> PILEKAP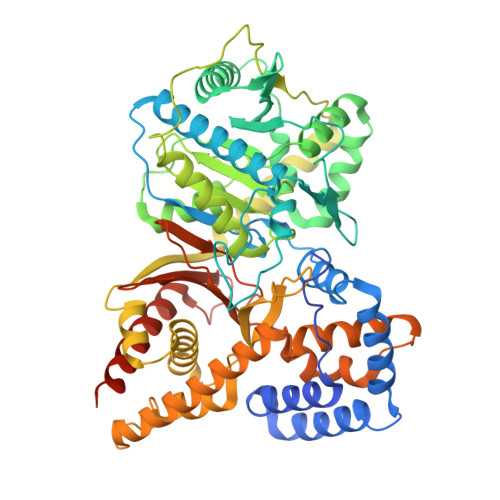QKMPVKASSWEELDLPKLPVPPLQQTLATYLQCMQHLVPEEQFRKSQAIVKRFGAPGGLGETLQEKLLERQEKTANWVSEYWLNDMYLNNRLALPVNSSPAVIFARQHFQDTNDQLRFAACLISGVLSYKTLLDSHSLPTDWAKGQLSGQPLCMKQYYRLFSSYRLPGHTQDTLVAQKSSIMPEPEHVIVACCNQFFVLDVVINFRRLSEGDLFTQLRKIVKMASNEDERLPPIGLLTSDGRSEWAKARTVLLKDSTNRDSLDMIERCICLVCLDGPGTGELSDTHRALQLLHGGGCSLNGANRWYDKSLQFVVGRDGTCGVVCEHSPFDGIVLVQCTEHLLKHMMTSNKKLVRADSVSELPAPRRLRWKCSPETQGHLASSAEKLQRIVKNLDFIVYKFDNYGKTFIKKQKYSPDGFIQVALQLAYYRLYQRLVPTYESASIRRFQEGRVDNIRSATPEALAFVQAMTDHKAAMPASEKLQLLQTAMQAQTEYTVMAITGMAIDNHLLALRELARDLCKEPPEMFMDETYLMSNRFVLSTSQVPTTMEMFCCYGPVVPNGYGACYNPQPEAITFCISSFHSCKETSSVEFAEAVGASLVDMRDLCSSRQPADSKPPAPKEKARGPSQAKQS> GPLGSVEQELATKMLQIQSKRFYLDVKQNRRGRFIKVAEIGADGRRSQIYLALSTAAEFRDHLSSFSDYYASLGPPNTDNLPEDGKLKSEMMIKDYRRYYLDLKENARGRFL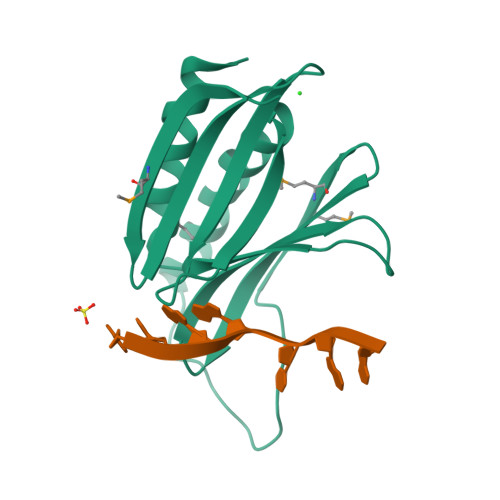RVSQTITRGGPRSQIALPAQGMIEFRDALTDLLEEFGAND>MKLWIDTDCGIDDATAILICLANPSIEIVGISCIGGNASLQNVIRNVNRTLKVWGKTDIPIFGGCQAPLVQPKMEIPHIHGGDGLGDINDNDFGTNTPNKLEKEHAVNALIHAANTIEDLNILCLAPLTNIAIALSMAPEAILKIKHFYIMGGAENGKGNITPYGEFNWRADPEAAQIVLQTYPQYQTTIASWTLAVFNSFNANDYDFFNLDGNLVRRFIRETWKPIIAFDGGRICPADPLAAFIAVYGDRAIKRAERLHL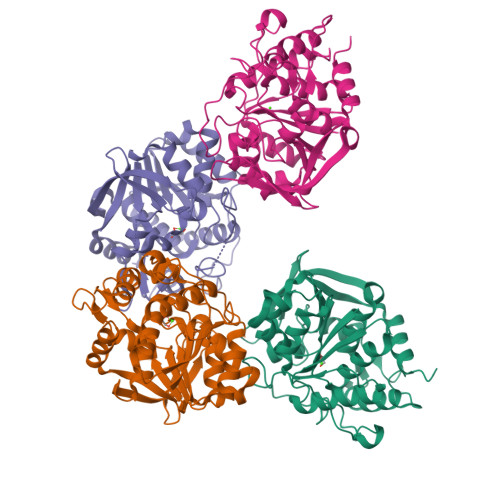SMVLEGEKLGMSLAEPDEKGCLVVKECDAELFVKILRELQDHQ[4x]>L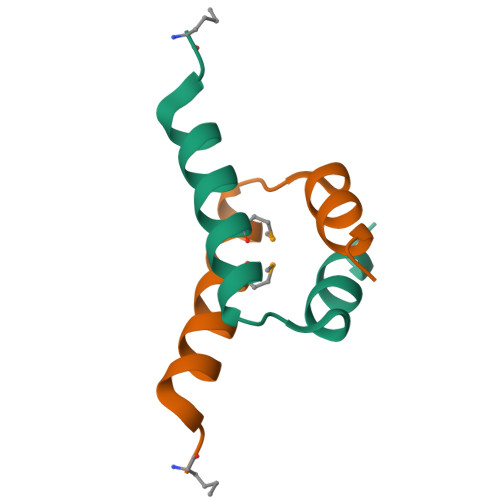VSKLSQLQTELMAALLESGLSKEALIQALGEW[2x]> MNLKALPAIEGDHNLKNYEETYRHFDWAEAEKHFSWHETGKLNAAYEAIDRHAESFRKNKVALYYKDAKRDEKYTFKEMKEESNRAGNVLRRYGNVEKGDRVFIFMPRSPELYFIMLGAIKIGAIAGPLFEAFMEGAVKDRLENSEAKVVVTTPELLERIPVDKLPHLQHVFVVGGEAESGTNIINYDEAAKQESTRLDIEWMDKKDGFLLHYTSGSTGTPKGVLHVHEAMIQQYQTGKWVLDLKEEDIYWCTADPGWVTGTVY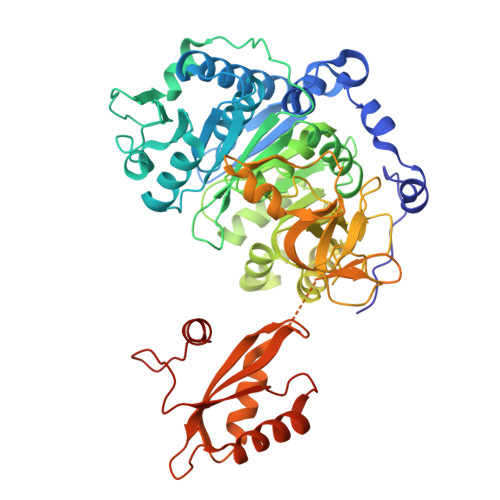GIFAPWLNGATNVIVGGRFSPESWYGTIEQLGVNVWYSAPTAFRMLMGAGDEMAAKYDLTSLRHVLSVGEPLNPEVIRWGHKVFNKRIHDTWWMTETGSQLICNYPCMDIKPGSMGKPIPGVEAAIVDNQGNELPPYRMGNLAIKKGWPSMMHTIWNNPEKYESYFMPGGWYVSGDSAYMDEEGYFWFQGRVDDVIMTSGERVGPFEVESKLVEHPAIAEAGVIGKPDPVRGEIIKAFIALREGFEPSDKLKEEIRLFVKQGLAAHAAPREIEFKDKLPKTRSGKIMRRVLKAWELNLPAGDLSTMED>[2x]MSLPMLQVALDNQTMDSAYETTRLIAEEVDIIEVGTILCVGEGVRAVRDL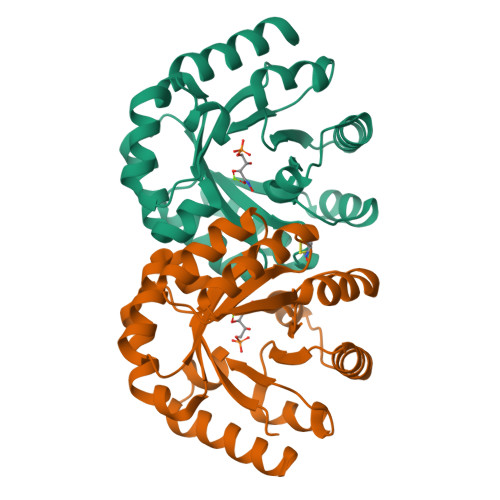KALYPHKIVLADAKIADAGKILSRMCFEANADWVTVICCADINTAKGALDVAKEFNGDVQIELTGYWTWEQAQQWRDAGIGQVVYHRSRDAQAAGVAWGEADITAIKRLSDMGFKVTVTGGLALEDLPLFKGIPIHVFIAGRSIRDAASPVEAARQFKRSIAELWG> MKVQAENAARLGRQV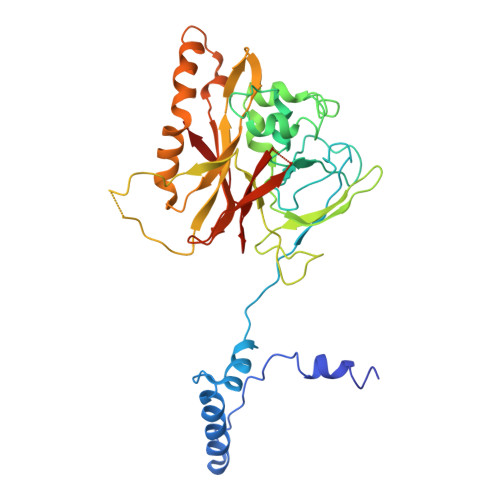LGLLPPPTHRVSLTRGPEFARGVRDLLSKYAASTRPTVGSLHEALRQAPFRQPTYGDFLVYSQTFSPQEPLGTFLFSFKQEDNGSSMDMLLTPTSLFMLSGMEAAKAPQTHKVAGVWYGSGSGLADFIPNLSELMDTGEFHTLLTPVGPMVQSVHSTFVTKVTSAMKGVGLARDEPRAHVGLTLPCDMLVDLDESCPMVQRREPAGLNVTIYASLVYLRVNQRPSMALTFFQSGKGFAEVVAMIKDHFTDVIRTKYIQLRHELYINRLVFGAVCTLGTVPFDSHPVHQSLNVKGTSLPVLVFANFEAACGPWTVFL FORMYCIN-5'-MONOPHOSPHATE | C10 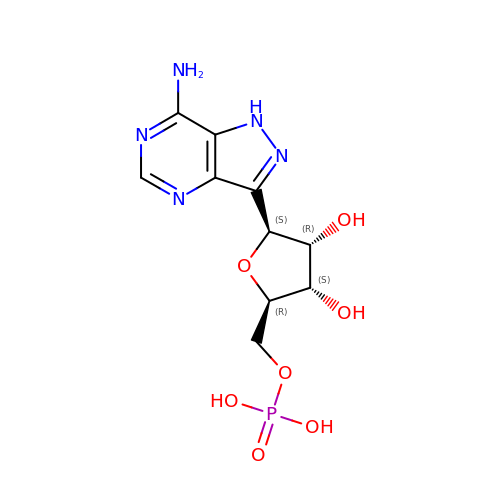H14 N5 O7 P | PBAHXXBYQACZMA-KSYZLYKTSA-N>MKRKLIVAVVCLIFICFGINTPAHATSVVSIPINNAGFEDPFIEVVDDYTVDTPPGWTTYNPNNLVPEKRTTWTSNNGVGYVGPGTQFYNQLAPEGRNIGYIYLAQKPGSGVAGFEQILDATLEPDTKYTLKVDVGNFGGEFQKISLAGFPGYRVELLAGDTVLAADHNNLYIKDGEFKTSTVTFTATPDNPYLDQKLGIRLIN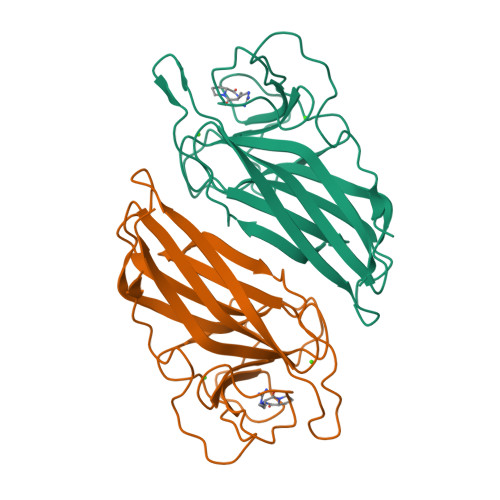LLQGTFSGLDFDNVRLTVEPAQT[4x]>MRGSHHHHHHGSVIFDKRIKDEEDVEKELGLPVLGSIQKFNMTNTRRSTSSLIVHEQPKSPISEKFRGIRSNIMFANPDSAVQSIVITSEAPGAGMSTIAANLAVAYAQAGYKTLIVDGDMRKPTQHYIFNLPNNEGLSSLLLNWSTYQDSIISTEIEDLDVLTSGPIPPNPSELITSRAFANLYDTLLMNYNFVIIDTPPVNTVTDAQLFSKFTGNVVYVVNSENNNKDEVKKGKELIEATGAKLLGVVLNRMPKDKSASYYAYYGTDES[2x]

We describe here the first crystal structure of a bacterial tyrosine kinase, namely CapB from the pathogen Staphylococcus aureus, in complex with the cytoplasmic domain of the transmembrane stimulatory protein CapA. CapA and CapB, among others, are involved as copolymerases in the synthesis of extracellular polysaccharides that are thought to be potent virulence factors. Reproducing the Gram-negative organization of BY-kinases by direct linkage of the Cap5A1Ct fragment (herein called CapACt) to the N-terminal extremity of Cap5B2 (herein called CapB) allowed the production of a fully active soluble protein called CapAB. The CapB kinase core possesses a P-loop type α/β mononucleotide binding fold.

The structure of the inactive P-loop CapAB(K55M) mutant was determined to 2.6Å resolution. It presents a subunit fold highly similar to that of the CapAB wild-type protein with an rmsd of 0.67 Å over 241 aligned residues. The major difference concerns the quaternary structure of this unphosphorylated form of the protein that associates to a ring-shaped octamer. The total surface contact area of about 2,000 Å between two neighbouring subunits is characteristic of biological interactions. Residues 216b–228b of the tyrosine cluster that were disordered in the phosphorylated wild-type structure form a long loop with Y225b side chain fitting in the active site of the neighbouring CapB molecule. The side chain of Y225b is bound in the active site of the neighbour subunit via hydrophobic sandwich interactions with the side chain of K82b and the two consecutive proline residues P159b–P160b forming an extended hhhhDTPP Walker B motif characteristic of the BY-kinase subfamily of P-loop ATPases. The hydroxyl group of Y225b is pointing toward the 4.8 Å distant β-phosphate of the bound ADP molecule. The catalytic residue D79b from the conserved DxD motif is positioned to deprotonate the Y225b hydroxyl, a prerequisite for its phosphorylation. Despite the absence of a nucleotide in the crystallization solution, ADP-Mg is observed in the P-loop of the CapAB(K55M) mutant protein. This is in agreement with a previous study showing that in P-loop proteins, this mutation inhibits the phosphate transfer but increases the affinity of the protein for the nucleotide.>GPGSATTVHGETVVNGAKLTVTKNLDLVNSNALIPNTDFTFKIEPDTTVNEDGNKFKGVALNTPMTKVTYTNSDKGGSNTKTAEFDFSEVTFEKPGVYYYKVTAEKIDKVPGVSYDTTSYTVQVHVLWNEEQQKPVATYIVGYKEGSKVPIQFKNSLDSTTLTV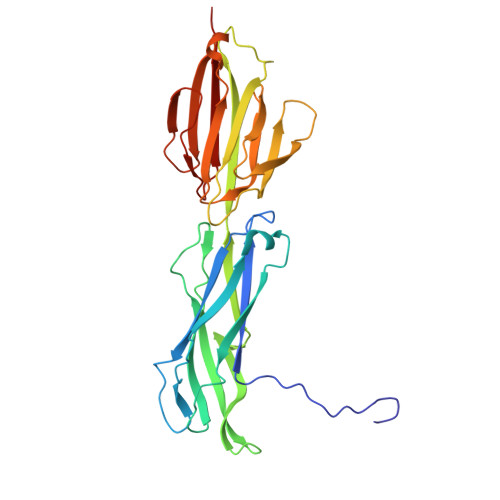KKKVSGTGGDRSKDFNFGLTLKANQYYKASEKVMIEKTTKGGQAPVQTEASIDQLYHFTLKDGESIKVTNLPVGVDYVVTEDDYKSEKYTTNVEVSPQDGAVKNIAGNSTEQETSTDKDMTITFTNKKVFE[3x]>[4x]MAKDIGINSDPNSSSVDKLMKSSGVSNPTYTLVWKVWILAVTLYYAIRIPLTLVFPSLFSPLLPLDILASLALIADIPLDLAFESRRTSGRKPTLLAPSRLPDLLAALPLDLLVFALHLPSPLSLLSLVRLLKLISVQASATRILSYRINPALLRLLSLVGFILLAAHGIACGWMSLQPPSENPAGTRYLSAFYWTITTLTTIGYGDITPSTPTQTVYTIVIELLGAAMYGLVIGNIASLVSKLDAAKLLHRERVERVTAFLSYKRISPELQRRIIEYFDYLWETRRGYEEREVLKELPHPLRLAVAMEIHGDVIEKVPLFKGAGEEFIRDIILHLEPVIYGPGEYIIRAGEMGSDVYFINRGSVEVLSADEKTRYAILSEGQFFGEMALILRAPRTATVRARAFCDLYRLDKETFDRILSRYPEIAAQIQELAVRRKELESSGLVPRGSVKHHHH

Here, we used SthK, a cyclic nucleotide-modulated channel from Spirochaeta thermophila, to define a ligand-gating trajectory that includes multiple on-pathway intermediates. cAMP is a poor partial agonist for SthK and depolarization increases SthK activity. CNG channels are tetrameric channels where each subunit consists of a voltage sensing domain (VSD, S1–S4), a pore domain (S5-S6), and a cytosolic cyclic nucleotide binding domain (CNBD) that is linked to the pore domain via a C-linker comprised of four α helices. Meanwhile, membrane depolarization increases cAMP-induced channel activity, suggesting that voltage modulates the agonist status of cAMP in SthK, similar to its action on other CNG channels, although the mechanism is not known. Cryo-EM structures of VSD mutants with increased activity yielded cAMP-bound closed states (identical to apo and cAMP-bound WT SthK), as well as four additional states: one gating intermediate and 3 open states with different degrees of opening.

Similarly, the sidechain of Arg120, another basic residue on the S4 helix, points into an electronegative pocket formed by Asp61, Ser80, Asp84, and Ser117 on the S2 and S3 helices. Removal of the positive charge of Arg120 would also weaken interactions between S4 and the neighboring helices, facilitating VSD movements in the membrane. In contrast to WT SthK and SthK Y26F, but in agreement with the higher open probability of SthK R120A, we also captured three open state conformations for SthK R120A. The C-linker/CNBD domains of these three states are all in the activated state, with the C-helix in contact with cAMP, the entire C-linker/CNBD assembly translated towards the membrane, rotated by about 12° with respect to the transmembrane region, and expanded radially with respect to the pore axis. The three additional conformations for SthK R120A all display open pores, albeit to different extents. We call them open states O1, O2, and O3, with O3 being the most open conformation (O1: 50037 particles, ~5%; O2: 149792 particles, ~14%; O3: 46629 particles, ~5%). The gradual increase of the pore radius from O1 to O2 to O3 is due to different endpoints of the S6 helix transitioning towards the final open state, O3, which suggests that O1 and O2 are on-pathway gating intermediates towards a fully open channel. In all three open conformations of SthK R120A, the lower two helical turns of the S4 helix of the VSD are displaced outwards by a small kink at Val118, allowing S5 to move, which creates space for the expansion of S6. The movements of S4 and S5 gradually increase among the three open conformations explaining the gradual increase in pore diameter (O1 < O2 < O3). For SthK R120A the open states are sufficiently stabilized relative to WT SthK and SthK Y26F on cryo-EM grids, possibly because of the further increased mean open dwell times.>[8x]SNAMNTTEFDGISHAEGLCDKEFIGKAISYLYRYGQIYIGKKIEPYGIGS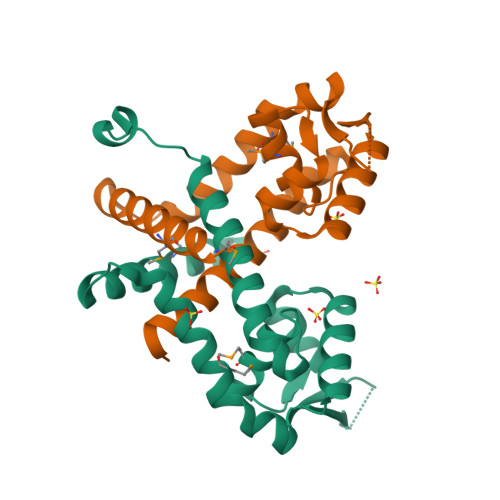GQFPFLMRLYREDGINQESLSDYLKIDKGTTARAIQKLVDEGYVFRQRDEKDRRSYRVFLTEKGKKLEPDMKKIASEWGEILFSSFDDRQRREITNSLEIMFENGLKIM>[6x]GSMNPEEKTVMLYNEYAEQAVLGSILTEPELIKECPLTPEHFSPGKHFNIYFTMQDLDRKGQSVDFTSIAARVGEKLPQLGGFGYLTELAASVASTTTFKQHCQTVSEYFQKRKAISIAQQIIENVNESDDGPVKPIQEAVSELMEIEASGTDDDDGSIDEALVTVYEEIESADGNITGVPSGFTELDRMTYGYKRRNFVLIAARPSMGKTAFALKQAKNMSDNDDVVNLHSLEMGKK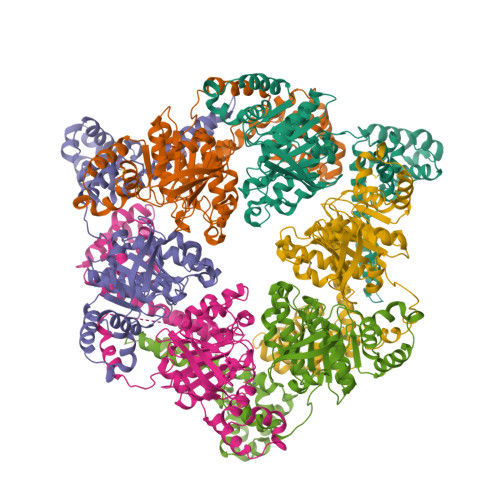ENIKRLIVTAGSINAQKIKAARRDFASEDWGKLSMAIGEISNSNINIFDKAGQSVNYIWSKTRQTKRKNPGKRVIVMIDYLQLLEPAKANDSRTNQISQISRDLKKMARELDVVVIALSQLSRQVEQRQDKRPMLSDLRESGQLEQDADIIEFLYRDDYYDKESESKNIVEVIIAKHRDGPVGTVSLAFIKEYGNFVNLERRFDDR>MIKKPEFGLMQPPKKRVRQELSEEQKQEIKEAFDLFDTNKTGSIDYHELKVAMRALGFDVKKPEILELMNE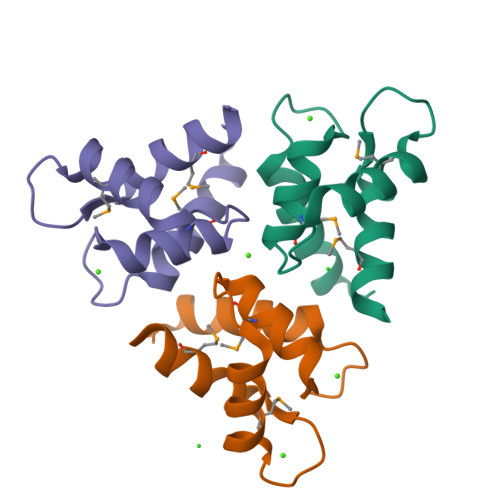YDREGNGYIGFDDFLDIMTEKIKN[3x]> PGVMTQEVGQLL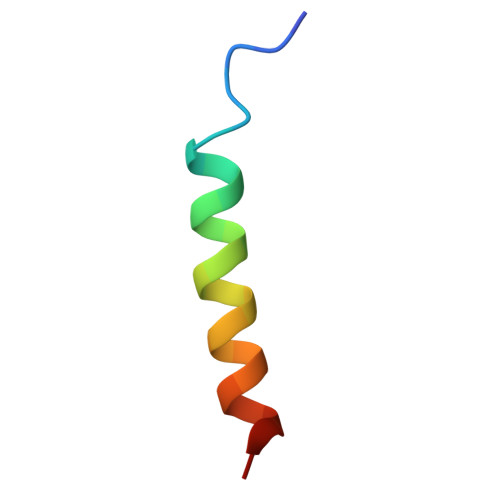QDMGDDVYQQYRSL>EFYHLVDDYGRGNGFFDKFNFFTGDDPTHGYVDYVSRDVAA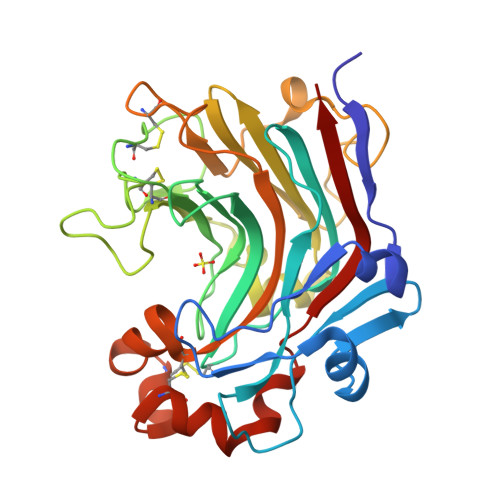GAGLIGERDGRTYMGVDFTNPASGRGRRSVRLESKNTYEHGLIVIDLAHMPGSVCGTWPAFWTLGTGDWPYGGAIDIIEGVNDNTFNHMVLHTSDGCTIDNDGFTGNLKTSNCYVYAPGQDANAGCGIEATDPNSYGKGFNSIGGGIYATEITPNGISIWFFPRGSEPGDVLGDNPNPANWDTPAAKFAGGGCDWEGKFNAQRLIFDVTFCGDWAGNVWGIGGCASRAANCVDFVRDNPSAFAESYWLVNSLRVYAP[2x]>MTDTLNPLVAAQEKVRIACEKLGCDPAVYELLKEPQRVIEISIPVKMDDGTVKVFKGWRSAHSSAVGPSKGGVRFHPNVNMDEVKALSLWMTFKGGALGLPYGGGKGGICVDPAELSERELEQLSRGWVRGLYKYLGDRIDIPAPDVNTNGQIMSWFVDEYVKLNGERMDIGTFTGKPVAFGGSEGRNEATGFGVAVVVRESAKRFGIKMEDAKIAVQGFGNVGTFTVKNIERQGGKVCAIAEWDRNEGNYALYNENGIDFKELLAYKEANKTLIGFPGAERITDEEFWTKEYDIIVPAALENVITGERAKTINAKLVCEAANGPTTPEGDKVLTERGINLTPDILTNSGGVLVSYYEWVQNQYGYYWTEAEVEEKQEADMMKAIKGVFAVADEYNVTLR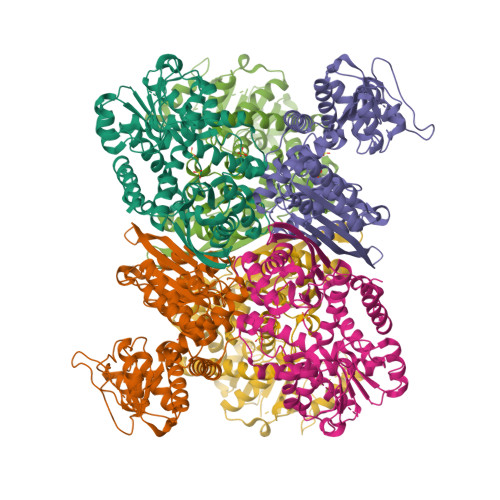EAVYMYAIKSIDVAMKLRGWY[2x]> QLTPTFYDNSCPNVS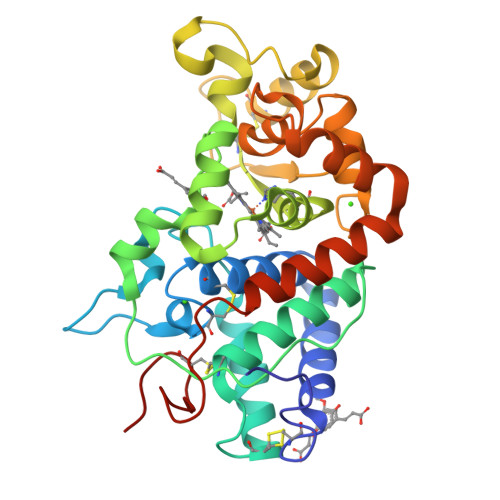NIVRDTIVNELRSDPRIAASILRLHFHDCFVNGCDASILLDNTTSFRTEKDAFGNANSARGFPVIDRMKAAVESACPRTVSCADLLTIAAQQSVTLAGGPSWRVPLGRRDSLQAFLDLANANLPAPFFTLPQLKDSFRNVGLNRSSDLVALSGGHSFGKNQCRFIMDRLYNFSNTGLPDPTLNTTYLQTLRGLCPLNGNLSALVDFDLRTPTIFDNKYYVNLEEQKGLIQSDQELFSSPNATDTIPLVRSFANSTQTFFNAFVEAMDRMGNITPLTGTQGQIRLNCRVVNSNS> MSLATGSVAPAITGIDLKGNS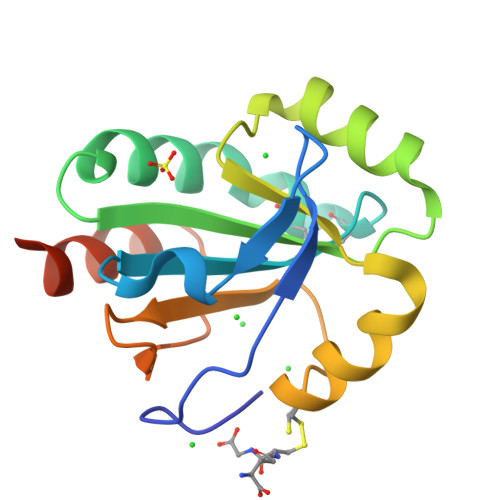VSLNDFKGKYVLVDFWFAGCSWCRKETPYLLKTYNAFKDKGFTIYGVSTDRREEDWKKAIEEDKSYWNQVLLQKDDVKDVLESYCIVGFPHIILVDPEGKIVAKELRGDDLYNTVEKFVNGAKEGHHHHHH Alpha-hydroxy acids are oxidized by a family of FMN-dependent enzymes. These enzymes use molecular oxygen to convert their substrate to product with the liberation of H2O2 as a by-product. PaLCTO is annotated as lactate oxidase and its closest homolog in Pediococcus acidilactici proteome does not use lactate as a substrate. We describe here structural and biophysical studies of PaLCTO, which revealed FMN-dependent folding and oligomerization of the enzyme.

We generated a mutant (A94G) based on literature precedent suggesting that the mutation of the residue may convert the enzyme to accept also larger substrates. The mutant was crystallized in the identical conditions as WT PaLCTO and the structure was determined at 2.0 Å resolution. The superimposition of the mutant and WT monomer structures showed high structural identity (rmsd = 0.16 Å for C-alpha 337 atoms). However, in the mutant structure we only observed the open conformation for the main polypeptide chain (loop 4: S201 –A219) and we were able to build the conformation completely with all the residues. Mutation of A94G likely reduces loop dynamics and therefore is completely resolved in the structure. The structures lay the ground for future biochemical experiments to determine the impact of mutation on loop dynamics.

> SMTMINGYEQSDREEKIDILNLESLEKQAEEIIPAGGFGYIAGGSEDEWTLKQNRMAFHHRQIAPKALSGIEKPELNTEIFGIPLNTPVMMAPAGAQGLAHSQGEKDTARGLAAVGGLMAQSTYSSVSIAETAAAGGDAPQFFQLYMSKDWNFNESLLDEAKKANVKAIILTVDATVDGYREADIKNKFTFPLPMANLIKFSEGNGQGKGIEEIYASAAQNIRPEDVKRIADYTNLPVIVKGIQTPEDAIRAIDAGAAGIYVSNHGGRQLNGGPASFDVLEDIATAVNKQVPIIFDSGVRRGSDVFKALASGADLVALGRPVIYGLALGGAKGVQSVFEHLNHELEIVMQLAGTKTIEDVKNNSLLNIKY>[8x]MKFRIGELADKCGVNKETIRYYERLGLIPEPERTEKGYRMYSQQTVDRLHFIKRMQELGFTLNEIDKLLGVVDRDEAKCRDMYDFTILKIEDIQ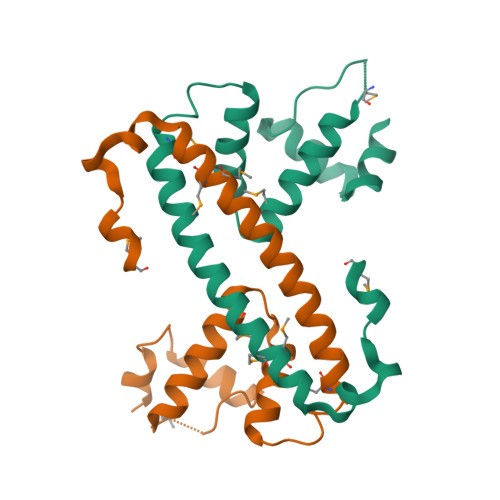RKIEDLKRIERMLMDLKERCPENKDIYECPIIETLMKK>[24x]XVQSKIGSLDNITHX

Functional tau is most abundant in neuronal axons where it binds to microtubules, assists microtubule assembly, and is essential for the structural integrity of neurons and for axonal transport. Here, we identify a new amyloidogenic segment, PAM4 (Polymorphic AMyloid segment in repeat 4), encompassing residues 350–362 of R4, and show that it self-assembles into amyloid fibrils. Cryo-EM revealed that PAM4 fibrils are highly polymorphic, and, remarkably, that the polymorphs formed by this segment in isolation recapitulate the conformations that PAM4 adopts in polymorphs from different human tauopathies. In all cases, the folds share a C-terminal β-strand (residues 358–362) but differ in the way they orientate the N-terminus about an intermediary GS-bend (residues 355–356).

We also determined the structure of PAM4 amyloid fibrils formed by a lower purity (92%) peptide batch. Two-dimensional (2D) classification revealed that this peptide batch also formed multiple fibril polymorphs, with three distinct PAM4 fibril structures that could be determined to high resolution. The remaining two PAM4 fibril structures were determined at resolutions of 2.7 Å (Type 3, 15% of the total population) and 2.9 Å (Type 4, 13% of the total population), respectively. The Type 3 and Type 4 fibrils share similar structural properties including crossovers around 80 nm and containing eight PAM4 subunits per layer of the fibril core, differing only in a slight re-positioning of the inter-protofilament interface. The resolution of the maps, in combination with liquid chromatography-mass spectrometry (LCMS) data, facilitated the identification of an adduct coming from a minor population of the peptide containing an N-terminal Fmoc protection group from peptide synthesis (~7.4%). Similarly, stacked protected N-termini pack at the protofibril interfaces of each of the three fibril structures with the C-termini extending towards the anterior fibril surface, which could potentially explain the additional structural morphologies resolved in the presence of the Fmoc protection group. Interestingly, the folds were interchangeable within the different fibril types, with Type 1 contaning FoldA and B, Type 2 fibrils containing FoldB, C and D, and Type 3 and Type 4 fibrils containing FoldC and D. Additionally, FoldC contains an intra-subunit salt bridge between K353 and D358 that stabilises its highly kinked (>90°) conformation. Specifically, the FoldC conformation of PAM4 stabilised by the K353-D358 salt-bridge is also found in tau C-fold protofilament polymorphs linked to Alzheimer’s disease (AD), Gerstmann-Sträussler-Scheinker (GSS), primary age-related tauopathy (PART) and cerebral amyloid angiopathy (CAA), while showing reasonable fit to chronic traumatic encephalopathy (CTE) polymorphs. Finally, FoldD PAM4 matches R2:R3:R4 (4R) tau strains that are associated with corticobasal degeneration (CBD) and argyrophilic grain disease (AGD).>[2x]MISILRRGLLVLLAAFPLLALAVQTPHEVVQSTTNELLGDLKANKEQYKSNPNAFYDSLNRI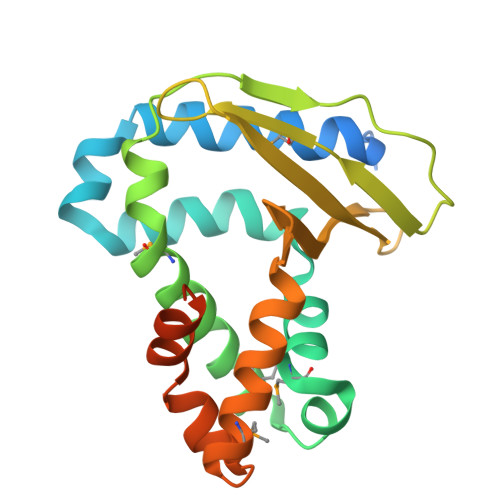LGPVVDADGISRSIMTVKYSRKATPEQMQRFQENFKRSLMQFYGNALLEYNNQGITVDPAKADDGKRASVGMKVTGNNGAVYPVQYTLENIGGEWKVRNVIVNGINIGKLFRDQFADAMQRNGNDLDKTIDGWAGEVAKAKQAADNSPEKSVKLEHHHHHH> APNDQHYREQWHYFDRYGVKADKVWDMGFTGQNVVVAVVDTGILHHRDLNANVLPGYDFISNSQISLDGDGRDADPFDEGDWFDNWACGGRPDPRK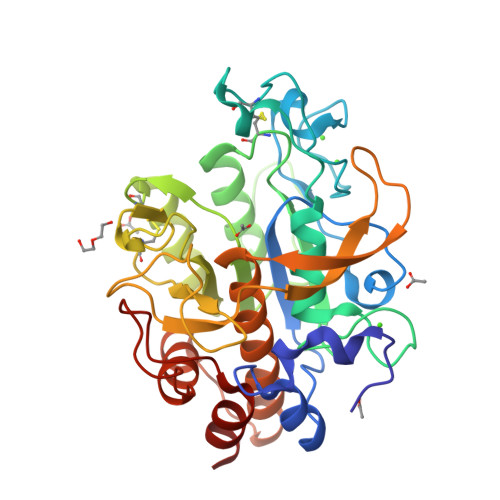ERSDSSWHGSHVAGTIAAVTNNRIGVAGVAYGAKVVPVRALGRCGGYDSDISDGLYWAAGGRIAGIPENRNPAKVINMSLGSDGQCSYNAQTMIDRATRLGALVVVAAGNENQNASNTWPTSCNNVLSVGATTSRGIRASFSNYGVDVDLAAPGQDILSTVDSGTRRPVSDAYSFMAGTSMATPHVSGVAALVISAANSVNKNLTPAELKDVLVSTTSPFNGRLDRALGSGIVDAEAAVNSVLG>MASGMIVTDAGADQPIVFVNRAFSTITGYAPNEVLGRNARFLQGPQTDPATVARLREAIAAARPIQERILNYRKDGQPFWNQLSISPVRDE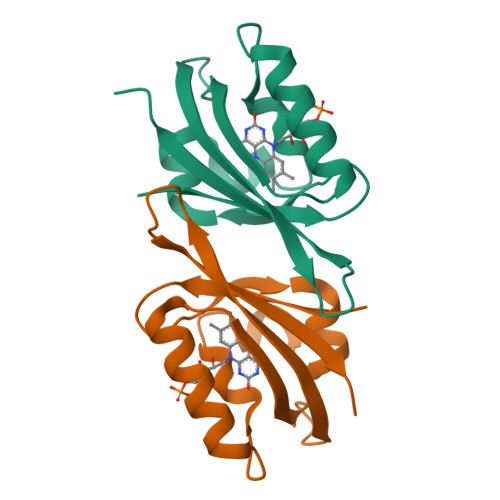TGNVVAFVGVQTDVTAHHHHHH[2x]>SNAREHDFDDLKFEHFLASAAGAFPAFLEVAEKRIIGEGVLRAVKESMRWHRAENVHFGAFLLLVPLISSWDAGGMVDIAEAARNRLRRTDFRDSLSVLEAFRLSNARVVEAGELNLKDRKTEEEIAQKKI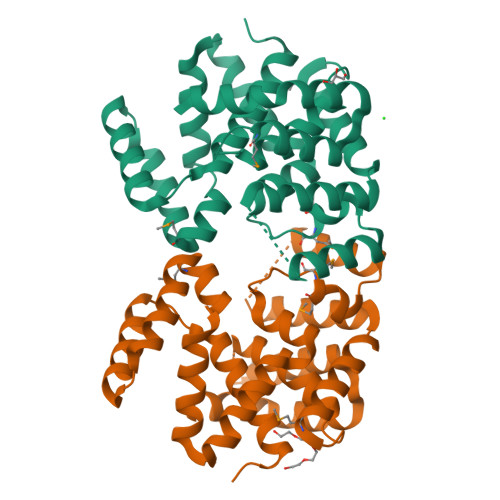NLYEWMKMAPEENLIARELVDGFKISIEGAKFLLSFGNSGKAVVELYYHLLSKFPDPLVIAKMGREYAEKITEWAEKARTEEERKELDEKLLKDGANPGTIADLTASSIFLALAEGWR[3x]> MGSSHHHHHHSSGPQQGLRYEAETA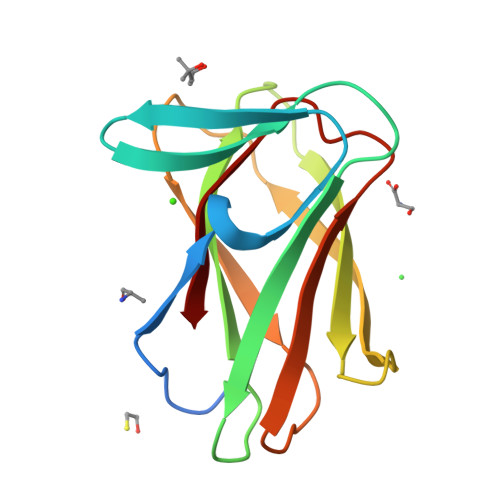TLKGKFRKKEHRKQTGVFFDKGKGNSIEWNISTGLAQVYALRFKYMNTTGKPMPVLMKFIDSKGVVLKEDILTFPETPDKWKMMSTTTGTFINAGHYKVLLSAENMDGLAFDALDI>MEDINFSSLAPRHGTRPFMGTWSDIGTSQLNGGAFNWSSLWSGLKNFGSTLKTYGSKAWNSTTGQALRDKLKEQNFQQKVVDGLASGINGVVDLANQAVQRQINSRLDPVPPAGSVEMPQVEEELPPLDKRGEKRPRPDAEETLLTHTDEPPPYEEAVKLGLPTTRPIAPLATGVLKPESNKPATLDLPPPASRPSTVAKPLPPVAVARARPGGSARPHANWQSTLNSIVGLGVQSVKRRRCY[12x];>[12x]MATPSMLPQWAYMHIAGQDASEYLSPGLVQFARATDTYFSLGNKFRNPTVAPTHDVTTDRSQRLTLRFVPVDREDNTYSYKVRYTLAVGDNRVLDMASTYFDIRGVLDRGPSFKPYSGTAYNSLAPKGAPNSSQWEQKKAGNGDTMETHTFGVAPMGGENITIDGLQIGTDATADQDKPIYADKTFQPEPQVGEENWQETESFYGGRALKKDTSMKPCYGSYARPTNVKGGQAKLKVGADGVPTKEFDIDLAFFDTPGGTVNGQDEYKADIVMYTENTYLETPDTHVVYKPGKDDASSEINLVQQSMPNRPNYIGFRDNFIGLMYYNSTGNMGVLAGQASQLNAVVDLQDRNTELSYQLLLDSLGDRTRYFSMWNQAVDSYDPDVRIIENHGVEDELPNYCFPLDGSGTNAAYQGVKVKNGNDGDVESEWENDDTVAARNQLCKGNIFAMEINLQANLWRSFLYSNVALYLPDSYKYTPANITLPTNTNTYDYMNGRVVPPSLVDAYINIGARWSLDPMDNVNPFNHHRNAGLRYRSMLLGNGRYVPFHIQVPQKFFAIKSLLLLPGSYTYEWNFRKDVNMILQSSLGNDLRTDGASISFTSINLYATFFPMAHNTASTLEAMLRNDTNDQSFNDYLSAANMLYPIPANATNVPISIPSRNWAAFRGWSFTRLKTKETPSLGSGFDPYFVYSGSIPYLDGTFYLNHTFKKVSITFDSSVSWPGNDRLLTPNEFEIKRTVDGEGYNVAQCNMTKDWFLVQMLAHYNIGYQGFYVPEGYKDRMYSFFRNFQPMSRQVVDEVNYKDYQAVTLAYQHNNSGFVGYLAPTMRQGQPYPANYPYPLIGKSAVTSVTQKKFLCDRVMWRIPFSSNFMSMGALTDLGQNMLYANSAHALDMNFEVDPMDESTLLYVVFEVFDVVRVHQPHRGVIEAVYLRTPFSAGNATT;> MMRRAYPEGPPPSYESVMQQAMAAAAAMQPPLEAPYVPPRYLAPTEGRNSIRYSELAPLYDTTRLYLVDNKSADIASLNYQNDHSNFLTTVVQNNDFTPTEASTQTINFDERSRWGGQLKTIMHTNMPNVNEFMYSNKFKARVMVSRKTPNGVTVTDGSQDILEYEWVEFELPEGNFSVTMTIDLMNNAIIDNYLAVGRQNGVLESDIGVKFDTRNFRLGWDPVTELVMPGVYTNEAFHPDIVLLPGCGVDFTESRLSNLLGIRKRQPFQEGFQIMYEDLEGGNIPALLDVDAYEKSKEESAAAATAAVATASTEVRGDNFASPAAVAAAEAAETESKIVIQPVEKDSKDRSYNVLPDKINTAYRSWYLAYNYGDPEKGVRSWTLLTTSDVTCGVEQVYWSLPDMMQDPVTFRSTRQVSNYPVVGAELLPVYSKSFFNEQAVYSQQLRAFTSLTHVFNRFPENQILVRPPAPTITTVSENVPALTDHGTLPLRSSIRGVQRVTVTDARRRTCPYVYKALGIVAPRVLSSRTF;>MSGSGSFEGGVFSPYLTGRLPSWAGVRQNVMGSTVDGRPVQPANSSTLTYATLSSSSVDAAAAAAAASAASAVRGMAMGAGYYGTLVANSSSTNNPASLNEEKLLLLMAQLEALTQRLGELTQQVAQLQEQTRAAVATVKSK[4x];> MQQQPPPDPAMRAALQSQPSGINSSDDWTQAMQRIMALTTRNPEAFRQQPQANRLSAILEAVVPSRSNPTHEKVLAIVNALVENKAIRGDEAGLVYNALLERVARYNSTNVQTNLDRMVTDVREAVAQRERFHRESNLGSMVALNAFLSTQPANVPRGQEDYTNFISALRLMVTEVPQSEVYQSGPDYFFQTSRQGLQTVNLSQAFKNLQGLWGVQAPVGDRATVSSLLTPNSRLLLLLVAPFTDSGSINRNSYLGYLINLYREAIGQAHVDEQTYQEITHVSRALGQDDPGNLEATLNFLLTNRSQKIPPQYTLSAEEERILRYVQQSVGLFLMQEGATPSAALDMTARNMEPSMYASNRPFINKLMDYLHRAAAMNSDYFTNAILNPHWLPPPGFYTGEYDMPDPNDGFLWDDVDSSVFSPRPGANERPLWKKEGSDRRPSSALSGREGAAAAVPEAASPFPSLPFSLNSIRSSELGRITRPRLLGEEEYLNDSLLRPEREKNFPNNGIESLVDKMSRWKTYAQEHRDDPSQGATSRGSAARKRRWHDRQRGLMWDDEDSADDSSVLDLGGSGNPFAHLRPRIGRMM;>MSKEIPTPYMWSYQPQMGLAAGAAQDYSTRMNWLSAGPAMISRVNDIRAHRNQILLEQSALTATPRNHLNPRNWPAALVYQEIPQPTTVLLPRDAQAEVQLTNSGVQLAGGATLCRHRPAQGIKRLVIRGRGTQLNDEVVSSSLGLRPDGVFQLAGSGRSSFTPRQAVLTLESSSSQPRSGGIGTLQFVEEFTPSVYFNPFSGSPGHYPDEFIPNFDAISESVDGYD[2x]

The ChAdOx1 viral vector, adapted from chimpanzee adenovirus Y25 (ChAd-Y25), is the basis for the ChAdOx1 nCoV-19 vaccine (AZD1222/Vaxzevria). We have determined the structure of the ChAdOx1 viral vector and used it in state-of-the-art computational simulations to demonstrate an electrostatic interaction mechanism with PF4, which was confirmed experimentally by surface plasmon resonance. Here, we characterized the capsid structure of ChAdOx1 and the primary receptor binding fiber knob protein. We have characterized its primary cell attachment protein, the fiber knob, and show that ChAdOx1, a simian adenovirus, shares considerable structural homology with human adenoviruses.

We have resolved the capsid structure of the ChAdOx1 viral vaccine vector to a resolution of 3.07 Å, the highest reported resolution of an adenovirus capsid to date. Determined at 3.07-Å resolution, ChAdOx1 has the quintessential icosahedral adenovirus capsid structure. The asymmetric unit contains the expected penton monomer; one peripentonal, two secondary, and one tertiary hexon trimers; one peripentonal and one secondary copy of Protein VIII; and partial density for the pIIIa protein. The pentameric penton protein, located at the 12 fivefold icosahedral vertices, had weaker signal, which could indicate a less well-ordered, or less stably interacting, protein than those observed in previous cryo-EM structures of HAdV-D26 and HAdV-C5. As in other reported structures, the penton RGD loop (residues 305 to 335), which is responsible for binding to integrins following attachment to the cell surface via the fiber knob protein, was left unmodeled because of the lack of signal, indicative of its flexibility. We observed partial densities for 12 copies of pVI in the base of the hexons that adopted two conformations, either wrapping around the hexon interior before extending into the capsid core or extending directly out of the base of the hexon to wrap over the top of pVIII. Hexon was well resolved, including the hypervariable regions (HVRs) on the exterior, enabling a complete reconstruction. ChAdOx1 is more electronegative than HAdV-D26 with negative charge extending into the interhexon spaces, while in HAdV-D26, it has electropositive charge in these regions. Results show freely diffusing PF4 frequently contacts the capsid surface of ChAdOx1 between the hexons, most commonly at the interfaces of three hexons where negative charge is concentrated, and the interhexon space is maximized. To identify amino acids that are potentially important for the ChAdOx1/PF4 interaction, we calculated the frequency of contacts between PF4 and the ChAdOx1 hexons in BD simulations. These indicate PF4 contacts residues in the HVRs of ChAdOx1.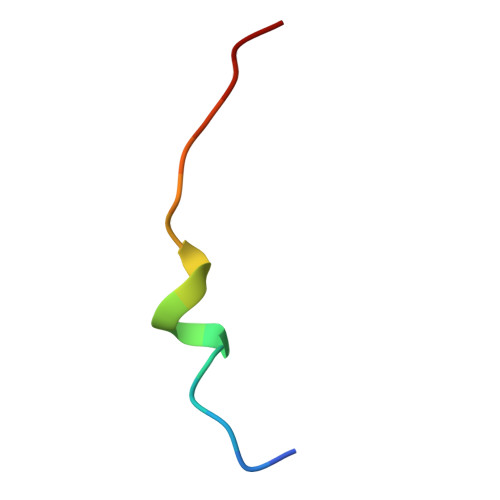> VSMAEEVLNLQLVSVQV6-chloranyl-2-oxidanylidene-N-[(1S,5R)-8-[4-[(phenylmethyl)amino]piperidin-1-yl]sulfonyl-8-azabicyclo[3.2.1]octan-3-yl]-1,3-dihydroindole-5-carboxamide | C28 H34 Cl N5 O4 S | 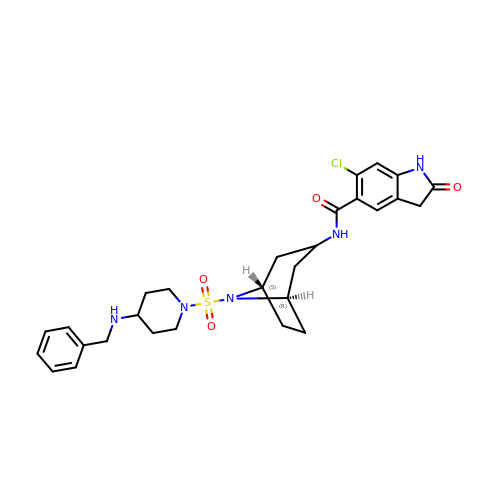SSDPURPCLGSTBN-NUNAXRQHSA-N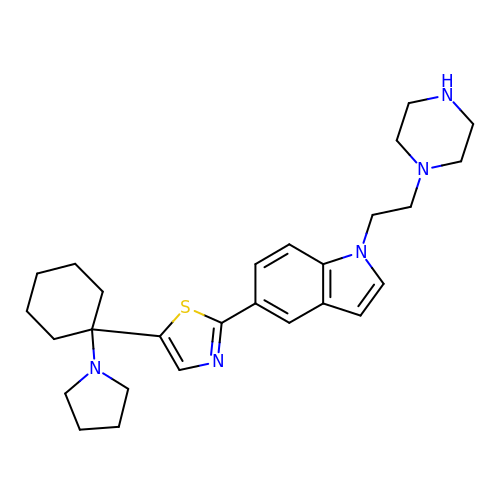1-[2-(piperazin-1-yl)ethyl]-5-{5-[1-(pyrrolidin-1-yl)cyclohexyl]-1,3-thiazol-2-yl}-1H-indole | C27 H37 N5 S | PWLNVBJHVGPQID-UHFFFAOYSA-N> AKPDRSSFVPSLFSKKKKNVTMRSIKTTRDRVPTYQYNMNFEKLGKCIIINNKNFDKVTGMGVRNGTDKDAEALFKCFRSLGFDVIVYNDCSCAKMQDLLKKASEEDHTNAACFACI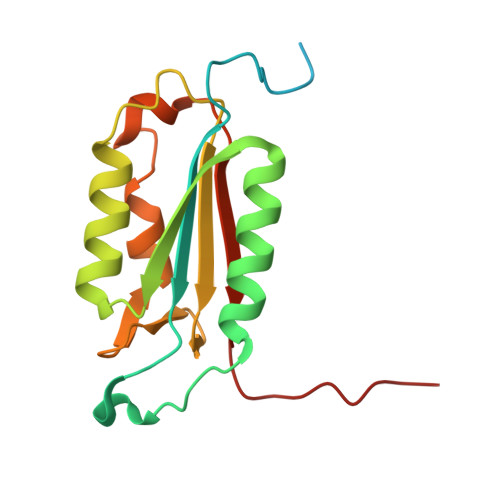LLSHGEENVIYGKDGVTPIKDLTAHFRGDRCKTLLEKPKLFFIQACRGTELDDGIQ> MVIFDEHKFRTLFPEFADPAAYPDVRLQMYFDIACEFISDRDSPYRILNGKALEACLYLLTAHLLSLSTMQVQGAAGGGVTAGGTQGGFITSATVGEVSVAKLAPPAKNGWQWW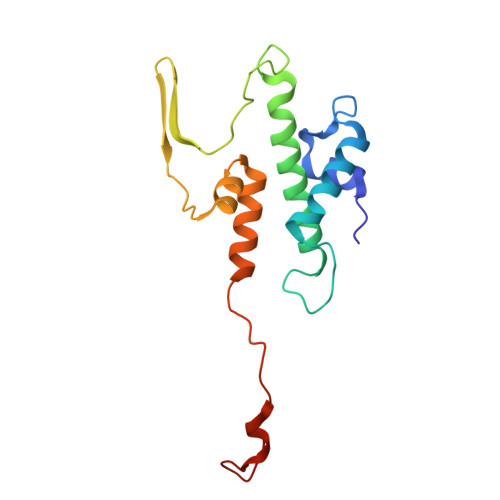LSGTPYGQELWALLSVKAVGGFYIGGLPERRGFRKVGGTFW> GTSSMADIGSRYSKISDNYSSLLQVSEALGRAGLESSNLIVGIDFTKSNEWTGAKSFNRKSLHHLSNTPNPYEQAITIIGRTLAAFDEDNLIPCYGFGDASTHDQDVFSFYPEGRFCNGFEEV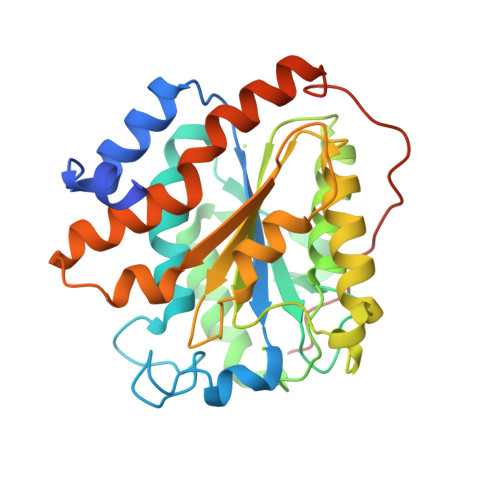LARYREIVPQLKLAGPTSFAPIIEMAMTVVEQSSGQYHVLVIIADGQVTRSVDTEHGRLSPQEQKTVDAIVKASTLPLSIVLVGVGDGPWDMMQEFADNIPARAFDNFQFVNFTEIMSKNKDQSRKETEFALSALMEIPPQYKATIELNLLGVRNGNIPQRIPLPPPVQSGSSFSSSR>IVGGYTCAANSIPYQVSLNSGSHFCGGSLINSQWVVSAAHCYKSRIQVRLGEHNIDVLEGNEQFINAAKIITHPNFNGNTLDNDIMLIKLSSPATLNSRVATVSLPRSCAAAGTECLISGWGNTKSSGSSYPSLLQCLKAPVLSDSSCKSSYPGQITGNMICVGFLEGGKDSCQGDSGGPVVCNGQLQGIVSWGYGCAQKNKPGVYTKVCNYVNWIQQTIAAN[3x];>KPGKCPVTYGQCLMLNPPNFCEMDGQCKRDLKCCMGMCGKSCVSPVK[2x]

SLPI (secretory leukocyte protease inhibitor) is a 107-residue protease inhibitor which inhibits various serine proteases, including elastase, cathepsin G, chymotrypsin and trypsin. The exact physiological function of SLPI has not been elucidated, but its major role is considered to be the protection of the airway epithelial surface from attached human neutrophil elastase which has been found in pulmonary lavage fluid and sputum from patients with inflammatory respiratory diseases. 1/2SLPI (recombinant C-terminal domain of SLPI Arg58–Ala107) has a potent inhibitory activity against multiple serine proteases such as trypsin, chymotrypsin, elastase, chymase and cathepsin G as that of intact SLPI. Generally, a main part of the affinity and inhibitory activity of the biological inhibitors depends on the P1 residue which penetrates deeply into the S1 pocket of the proteases.

The present work describes the first X-ray structure analyses of 1/2SLPI with P1 Leu residue with trypsin (PPT) at 2.0 Å and comparisons are made with the previously reported 1/2SLPI–HNE and SLPI–chymotrypsin complex structures. Two complexes (one with chains A and B, the other with chains C and D) appear to interact with the reversible inhibition mechanism. Additionally, one uncomplexed PPT molecule (chain E) exists per asymmetric unit. Two independent 1/2SLPI molecules are superposing each other at the corresponding main-chain (Lys60i–Lys106i) atoms and the root-mean-square difference (RMSD) is 0.19 Å. The RMSD value among three independent PPT molecules was 0.35 Å by superposing with the corresponding main-chain atoms between residues Ile16 and Asn245. In all complex structures (1/2SLPI–PPT, 1/2SLPI–HNE and SLPI–chymotrypsin), the Leu72i residue of 1/2SLPI is located in the S1 pocket as a P1 residue. The primary binding region appears to range from P3 Gln70i to P2′ Leu74i by intermolecular hydrogen bonds. In the 1/2SLPI–PPT complex, the S5 pocket of PPT formed by residues Tyr217 and Lys224 interacts with the P5 Tyr68i residue of 1/2SLPI. As the enzymes have not drastically changed the structure of the S5 site by 1/2SLPI binding, 1/2SLPI should change the P5 Tyr68i conformation to accommodate each S5 pocket. 1/2SLPI controls the inhibitory activity by using moieties from P2′ to P5 and can be adapted to various proteases flexibly.> E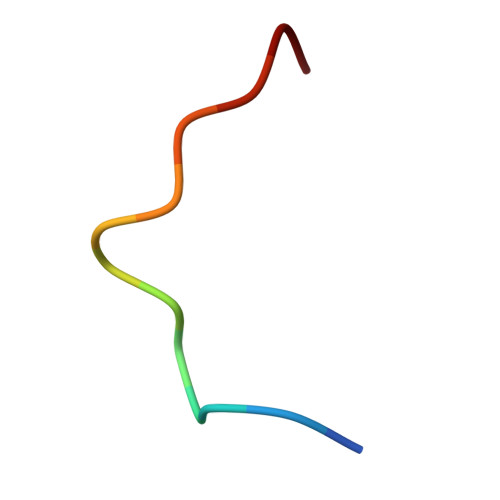DSILQPGAFSAN> GGAGCGUCGUGUCUCUUGUACGUCUCGGUCACAAUACACGGUUUCGUCCGGUGCGUGGCAAUUCGGGGCACAUCAUGUCUUUCGUGGCUGGUG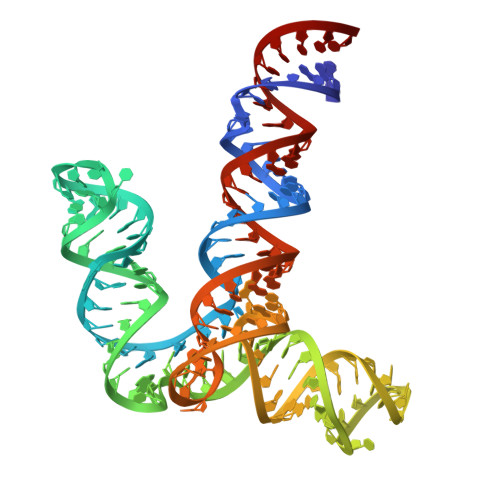UGACCGCGCAAGGUGCGCGCGGUACGUAUCGAGCAGCGCUCC>GPLGSLLETKASYLCDVAGAEVVRQFLDQYFRIFDSGNRQALLDAYHEKAMLSISMPSASQAGRLNSFWKFNRNLRRLLNGEENRTRNLKYGRLACVSTLDEWPKTQHDRRTFTVDLTIYNTSMMVFTVTGLFKELNDETNNPASMELYDVRHFARTYVVVPQNNGFCIRNETIFITNATHEQVREFKRSQ[2x];>GSMDSDLKAKVESCARTADTFTRLYYASVDNRRQ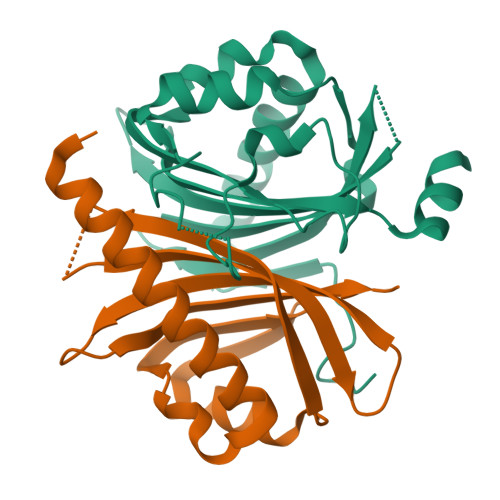QIGRLYLDNATLSWNGNGAIGRQMIESYFQELPSSNHQLNTLDAQPIVDQAVSNQLAYLIMASGSVKFADQQLRKFQQTFIVTAENDKWKVVSDCYRMQEV[2x]Synpcc7942_2462 from the cyanobacteria Synechococcus elongatus PCC 7942 encodes a putative sugar kinase (SePSK), and this kinase contains 426 amino acids. The At2g21370 gene product from Arabidopsis thaliana, xylulose kinase-1 (AtXK-1), whose mature form contains 436 amino acids, is located in the chloroplast (ChloroP 1.1 Server). SePSK and AtXK-1 display a sequence identity of 44.9%, and belong to the ribulokinase-like carbohydrate kinases, a sub-family of FGGY family carbohydrate kinases. Domain I exhibits a ribonuclease H-like folding pattern, and is responsible for the substrate binding, while domain II possesses an actin-like ATPase domain that binds cofactor ATP.

We therefore used single isomorphous replacement anomalous scattering method (SIRAS) for successful solution of the apo-SePSK structure at a resolution of 2.3 Å. Subsequently, the apo-SePSK structure was used as molecular replacement model to solve all other structures identified in this study. Our structural analysis showed that apo-SePSK consists of one SePSK protein molecule in an asymmetric unit. The amino-acid residues were traced from Val2 to His419, except for the Met1 residue and the seven residues at the C-termini. Apo-SePSK contains two domains referred to further on as domain I and domain II. In the SePSK structure, B1 and B2 are sandwiched by A1, A2 and A3, and the whole structure shows the A1/B1/A2/B2/A3 (α/β/α/β/α) folding pattern, which is in common with other members of FGGY family carbohydrate kinases. The overall folding of SePSK resembles a clip, with A2 of domain I acting as a hinge region. As a consequence, a deep cleft is formed between the two domains. After comparing structures of apo-SePSK, RBL-SePSK and AMP-PNP-SePSK, we noticed that these structures presented here are similar. Since the two domains of SePSK are widely separated in this structure, we hypothesize that our structures of SePSK represent its open form, and that a conformational rearrangement must occur to switch to the closed state in order to facilitate the catalytic process of phosphorylation of sugar substrates.

> MGMVVALGLDFGTSGARAIACDFDSDRSVSVSVTFPKTSQNWPQVWREALWQLLTQIPADWRSRIERIAIDGTSGTVLLCDREGQPQTEPLLYNQACPIDLADLADWVPADHAALSSTSSLAKLWFWQQQFGALPPDWQILAQADWLSLQLHGCSQQSDYHNALKLGYSPDRERFSKNLLDSELGALLPVVHEPGVAIGPILPAIAQEFGLSPDCQICAGTTDSIAAFLASGAHQPGEAVTSLGSTIVLKLLSQVAVSDRLTGVYSHKLGGYWLTGGASNCGGATLRQFFPDTELESLSCQIDPTKKSGLDYYPLPSRGERFPIADPDRLPQLEPRPENPVQFLQGLLEGLTQVETLGYQRLQDLGATPLKRIWTAGGGAKNAVWQQLRQQAIGVPIAIAPNTEAAFGTARLAAFGLAAFHSAGLKRTLEHHHHHH>[3x]MDYKDHDGDYKDHDIDYKDDDDKLEVLFQGPGSMATPSMMPQWAYMHIAGQDASEYLSPGLVQFARATDTYFSMGNKFRNPTVAPTHDVTTDRSQRLMLRFVPVDREDNTYSYKVRYTLAVGDNRVLDMASTFFDIRGVLDRGPSFKPYSGTAYNSLAPKGAPNTSQWIVTTNGDNAVTTTTNTFGIASMKGDNITKEGLQIGKDITTTEGEEKPIYADKTYQPEPQVGEE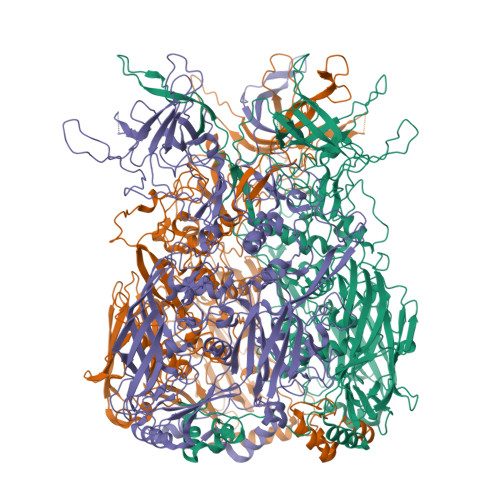SWTDTDGTNEKFGGRALKPATNMKPCYGSFARPTNIKGGQAKNRKVKPTTEGGVETEEPDIDMEFFDGRDAVAGALAPEIVLYTENVNLETPDSHVVYKPETSNNSHANLGQQAMPNRPNYIGFRDNFVGLMYYNSTGNMGVLAGQASQLNAVVDLQDRNTELSYQLLLDSLGDRTRYFSMWNQAVDSYDPDVRIIENHGIEDELPNYCFPLNGIGPGHTYQGIKVKTDDTNGWEKDANVAPANEITIGNNLAMEINIQANLWRSFLYSNVALYLPDVYKYTPPNITLPTNTNTYEYMNGRVVSPSLVDSYINIGARWSLDPMDNVNPFNHHRNAGLRYRSMLLGNGRYVPFHIQVPQKFFAVKNLLLLPGSYTYEWNFRKDVNMVLQSSLGNDLRTDGATISFTSINLYATFFPMAHNTASTLEAMLRNDTNDQSFNDYLSAANMLYPIPANATNIPISIPSRNWAAFRGWSFTRLKTKETPSLGSGFDPYFVYSGSIPYLDGTFYLNHTFKKVSIMFDSSVSWPGNDRLLSPNEFEIKRTVDGEGYNVAQCNMTKDWFLVQMLANYNIGYQGFYIPEGYKDRMYSFFRNFQPMSRQVVDEVNYTDYKAVTLPYQHNNSGFVGYLAPTMRQGEPYPANYPYPLIGTTAVKSVTQKKFLCDRTMWRIPFSSNFMSMGALTDLGQNMLYANSAHALDMTFEVDPMDEPTLLYLLFEVFDVVRVHQPHRGVIEAVYLRTPFSAGNATT> GSMEISIDALMAKIKSTMMTREQIQKEYDALVKS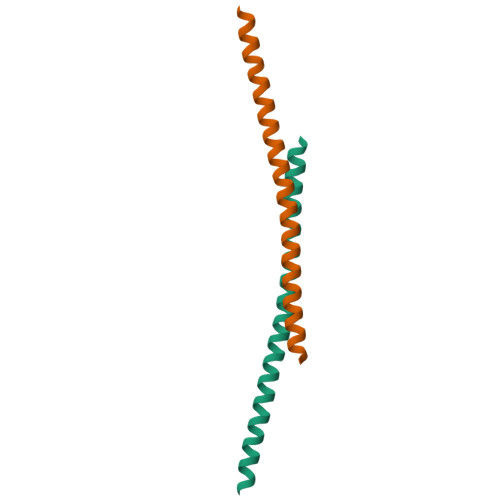SEDLLSALQKKKQQEEEAERLRRIQEEMEKERKRR> GGCUUAUCAAGAGAGGGCGAGCGACUGGCGCGAAGACCCCCGGCAACCAGAAAUGGUGCCAAUUCCUGCAGCGGAAACGUUGAAAGAUGAGCCG

One especially common junction element is the kink-turn (k-turn). k-turns are elements in double-stranded RNA that introduce a tight kink into the helical axis, with an included angle close to 50°. A standard k-turn comprises a three-nucleotide bulge followed by successive G•A and A•G trans G(sugar edge)•A(Hoogsteen edge) basepairs. k-turns are commonly-occurring motifs that introduce sharp kinks into duplex RNA, thereby facilitating tertiary contacts. Both the folding and conformation of k-turns are determined by their local sequence. k-turns fall into two conformational classes, called N3 and N1, that differ in the pattern of hydrogen bonding in the core. We show here that this is determined by the basepair adjacent to the critical G•A pairs.

We therefore decided to extend the study with a systematic structural analysis of HmKt-7 as a function of the 3b,3n sequence. This was performed in the constant environment of the SAM-I riboswitch, modified by replacing its natural k-turn by HmKt-7 with different 3b,3n sequences. In this way we could observe the effect of changing the 3b,3n sequence alone in an otherwise completely unchanged RNA molecule. Altogether seven of the new structures are in the N1 conformation, and clearly simply changing the 3b,3n sequence alone is sufficient to induce the structure of Kt-7 to change within the riboswitch environment. The N3 group contain a preponderance of 3b,3n = A•G and U•U pairs, and the N1 group comprise mainly 3b,3n = U•G, C•A and C•C pairs. We note the majority (6/8) of the 3b = pyrimidine k-turns form N1 structures. Evidently the 3b,3n sequence is the major determinant of the k-turn conformation.> TTHFSIVDKDGNAVSNTYTLNWDFGSGVVVKGAGFLLNDEMDDFSSKPGVANAFGVVGSDANAIEPGKRMLSSMSPSIVTRDGHVSLVLGTPGGSRIFTSIFQVLNNVYDFHLPLEKAVAAQRVH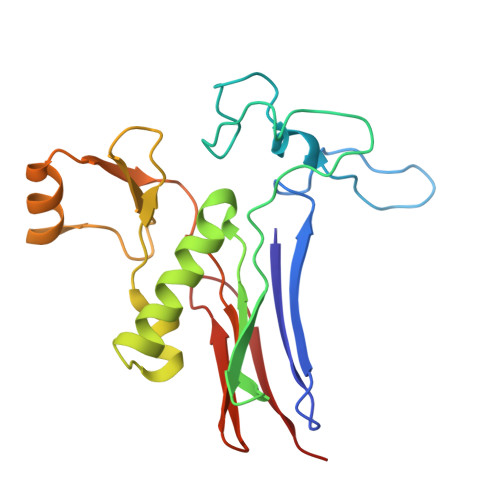HQLLPKDTIYYDAYAPLTGKVADELKAMGYTLEDQGDNMGDIQAIRVNGKALETASDPRGRGVGMVVKP4-[2-(trifluoromethyl)benzoyl]piperazin-2-one | 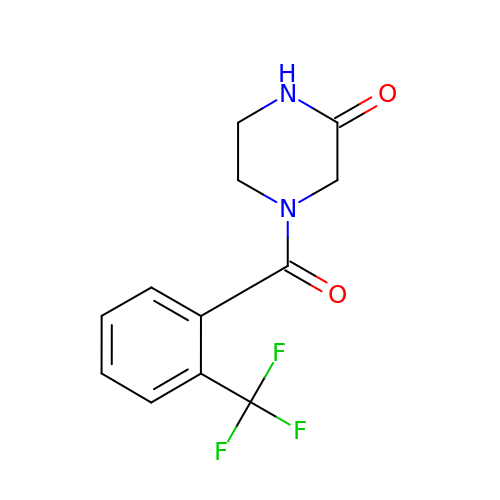C12 H11 F3 N2 O2 | JQOVYBILMPXMLQ-UHFFFAOYSA-N Hybrid clusters are metallo-cofactors constituted of a mixture of Fe atoms bridged with sulphur and oxygen atoms. The most notorious enzymes harbouring them as a prosthetic group are the hybrid cluster proteins (HCPs, also historically named prismane protein), which are present in strict or facultative anaerobic archaea and bacteria [e.g., the bacterium Desulfovibrio vulgaris and the archaeon Pyrococcus furiosus], and even a few unicellular eukaryotes [e.g., the microalga Chlamydomonas reinhardtii]. More recently, the HCP was shown to act as high-affinity nitric oxide (NO)-reductase, detoxifying NO into nitrous oxide N2O at physiological concentrations, and its overexpression protects cells against nitrosative stress. MtHCP is a monomeric 548-amino acid peptide organised in three domains (first domain residues 1–222, second domain 223–368, and third domain 369–548) harbouring a cubane [4Fe-4S] cluster and the hybrid cluster.

The native HCP from the thermophilic methanogen M. thermolithotrophicus (MtHCP) was purified anaerobically by multiple chromatography steps and immediately crystallised without freezing. The crystal structure was solved by single-wavelength anomalous dispersion at the Fe K-edge (SAD) and refined to a 1.45-Å resolution. Based on the nomenclature, MtHCP would belong to class I, coherently with cluster binding motif and its monomeric state confirmed in the crystal structure. The structure harbours a hybrid cluster in a [4Fe-3S] composition, matching the bacterial homologues in their reduced state. The active sites of MtHCP and the 1.25-Å resolution structure of the reduced DdHCP are superimposable. The main difference is a 1.0-Å shift of the “Y-atom” at the hybrid cluster vicinity, which has also been attributed to an oxygen atom in MtHCP based on the electron density. Because of the unequivocal chemical composition [4Fe 2μ3-S μ2-S (O)] of the hybrid cluster, we propose that the as-isolated MtHCP represents the reduced state (the nomenclature MtHCPred will be used below). A cavity analysis by the CAVER programme showed that the hydrophobic channels are also present in the MtHCPred structure. Five channels devoid of any water molecules were detected, spanning an overall distance of approximately 63-Å (tunnel length from the extremities of tunnels 1 and 5) within the enzyme from an edge to another. The channelling system connects the active site to several openings on the protein surface, and most of the side chains structuring the channels are hydrophobic (57/62), probably for repelling charged or polar molecules that would disturb the reaction.

> MRPSKMFCYQCQETAKNTGCTIIGVCGKKDNVANLQDLLVYTVKGLAVVRENLGYSNDKTDRYIVDALFTTITNVNFDDKDIIEKIKEGLALREEAASKSTCPGCGGDLPDCATWTADSDDEIIKKANSLEVSVLATENEDVRSLRELLTYGVKGIAAYLHHAMVLGYDNKDIHKFIRKALVATTDDSLSADELTALVLECGKYAVDTMALLDKANTETYGHPEITEVDIGVRNNPGILISGHDLKDLEQLLEQTKGTGVDVYTHSEMLPAHYYPAFKKYDHFVGNYGGSWWRQKEEFEAFNGPIVMTTNCLVPPAESYKDRIYTTGVVGFPGLKRIPEDENGNKDFSEVIEQAKKCAPPKQLETGKIVGGFAHNQVLALADKVVEAVKSGAIRKFVVMAGCDGRHPSREYYTEFAKKLPNDTVILTAGCAKYRYNKLGLGDIGGIPRVLDAGQCNDCYSLAVIALKLKEVFELDDINDLPIAFNVAWYEQKAVAVLLALLYLGVKDIVLGPTLPAFLSPNVAKVLVEKFGISGITTVDEDIERLINK Alkaline Phosphatase (AP) and other nonspecific phosphatases are some of Nature's most impressive catalysts, achieving preferential transition state over ground state stabilization of more than 1022-fold while utilizing interactions with only the five atoms attached to the transferred phosphorus. The AP active site contains three divalent metal ions and additional positively charged side chains in position to interact with the negatively charged phosphate monoester substrate. We tested a model that AP achieves a portion of this preference by destabilizing ground state binding via charge repulsion between the anionic active site nucleophile, Ser102, and the negatively charged phosphate monoester substrate. The results show that the Pi trianion binds with an exceptionally strong femtomolar affinity in the absence of Ser102, show that its binding is destabilized by ≥108-fold by the Ser102 alkoxide, and provide direct evidence for ground state destabilization.

To reduce the Pi affinity of the Ser102 mutants to a measurable range, an additional mutation was introduced. Previous studies showed that mutation of Arg166, which interacts with two of the phosphoryl oxygen atoms, reduces Pi binding affinity by ∼103-fold at pH 8.0 ( = 460 µM and  = 640 µM,;  = 0.5–1 µM,). When Ser102 was mutated in the R166S AP background, Pi binding was observed using the equilibrium-binding assay with dissociation constants of 66 and 77 nM for S102G/R166S and S102A/R166S AP, respectively, at pH 8.0. The mutations that remove Ser102 increase affinity by ∼103-fold, providing additional strong support for a destabilizing influence of Ser102. However, the orientation of Pi bound to WT AP and the Ser102Gly and Ala mutants is indistinguishable. The Pi binding geometry in the S102G/R166S AP double mutant, solved herein (see Table S2 for refinement statistics), is also indistinguishable from that in WT AP. A comparison of our newly obtained S102G/R166S AP structure to a previously obtained structure of R166S AP also reveals another active site property, an interplay between Ser102 and Arg166 in positioning bound Pi that underscores the role of Arg166 in specifically stabilizing the transition state. Comparisons of X-ray crystal structures of AP with and without Ser102 reveal the same active site and Pi binding geometry upon removal of Ser102, suggesting that the destabilization does not result from a major structural rearrangement upon mutation of Ser102. The observed Pi binding affinity of S102G/R166S AP remains constant above pH 7. This dependence is different than that for WT and R166S AP, indicating that the protonation event(s) involved in Pi binding to S102G/R166S AP differ from those when Ser102 is present. Thus, S102G/R166S AP binds preferentially to , presumably by virtue of the increased negative charge of and the stronger net interactions with the positively charged AP active site.

>[2x]MPVLENRAAQGDITAPGGARRLTGDQTAALRDSLSDKPAKNIILLIGDGMGDSEITAARNYAEGAGGFFKGIDALPLTGQYTHYALNKKTGKPDYVTDGAASATAWSTGVKTYNGALGVDIHEKDHPTILEMAKAAGLATGNVSTAELQDATPAALVAHVTSSKCYGPSATSEKCPGNALEKGGKGSITEQLLNARADVTLGGGAKTFAETATAGEWQGKTLREQAQARGYQLVSDAASLNSVTEANQQKPLLGLFADGNMPVRWLGPKATYHGNIDKPAVTCTPNPQRNDSVPTLAQMTDKAIELLSKNEKGFFLQVEGASIDKQDHAANPCGQIGETVDLDEAVQRALEFAKKEGNTLVIVTADHAHASQIVAPDTKAPGLTQALNTKDGAVMVMSYGNSEEDSQEHTGSQLRIAAYGPHAANVVGLTDQTDLFYTMKAALGL> MTISSAHPETEPKWWKEATFYQIYPASFKDSNDDGWGDMKGIASK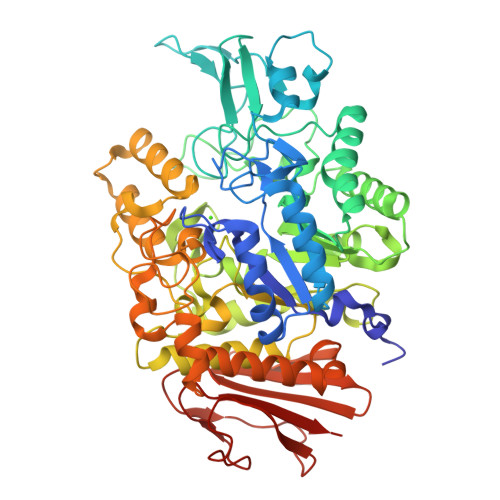LEYIKELGADAIWISPFYDSPQDDMGYDIANYEKVWPTYGTNEDCFALIEKTHKLGMKFITDLVINHCSSEHEWFKESRSSKTNPKRDWFFWRPPKGYDAEGKPIPPNNWKSYFGGSAWTFDEKTQEFYLRLFCSTQPDLNWENEDCRKAIYESAVGYWLDHGVDGFRIDVGSLYSKVVGLPDAPVVDKNSTWQSSDPYTLNGPRIHEFHQEMNQFIRNRVKDGREIMTVGEMQHASDETKRLYTSASRHELSELFNFSHTDVGTSPLFRYNLVPFELKDWKIALAELFRYINGTDCWSTIYLENHDQPRSITRFGDDSPKNRVISGKLLSVLLSALTGTLYVYQGQELGQINFKNWPVEKYEDVEIRNNYNAIKEEHGENSEEMKKFLEAIALISRDHARTPMQWSREEPNAGFSGPSAKPWFYLNDSFREGINVEDEIKDPNSVLNFWKEALKFRKAHKDITVYGYDFEFIDLDNKKLFSFTKKYNNKTLFAALNFSSDATDFKIPNDDSSFKLEFGNYPKKEVDASSRTLKPWEGRIYISE>[7x]APAANDSSQATLNFSGRVTSSLCQVKTDDLVKNISLGEVSKSALEATGKSPAQSFQVNLINCDSLTDDISYVLADANNNGTTTAYLVP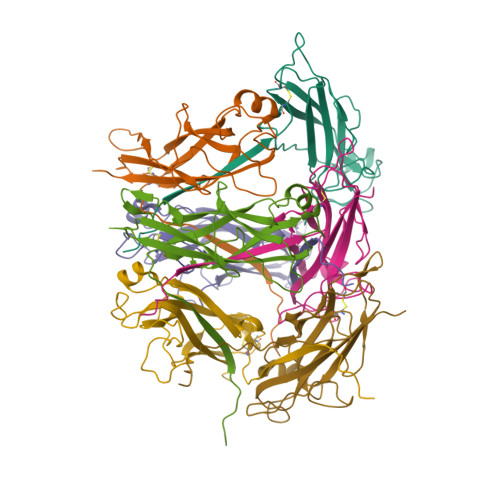KSGDTAATGVGVFVETSKGTPVNIGSDQKLDVVANKGNALSEQVIPLRAYIGTQTRAAGAIGTDVTAGTVDATGVLTIRAADAT> MAHHHHHHMTALLIRNVRTGADDALDILIEGDRIARTGPSLDAPPGCAIEEGAGAIALPGLVEGHTHLDKTHWGMPWYRNAVGPRLVDRIENERHYRATSGHDAGAASLALARAFLAAGTTRIRTHVDVDTDAGLRHLHRVL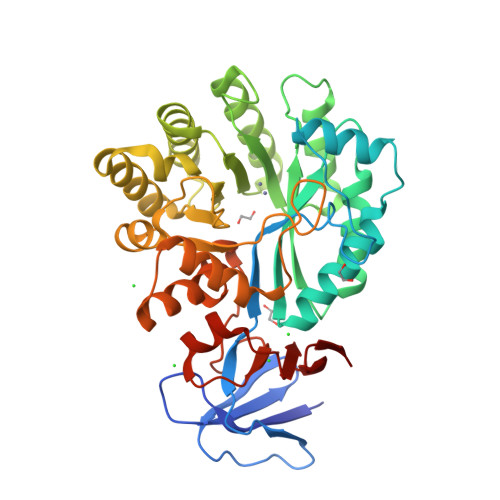DTRETLRGQVEIQIVAFPQSGVLKRPGTDALLADALAAGADLLGGLDPCAIEGDPVKAVDVLFGIAERYGRGLDLHLHERGSMGAYSLDLILQRTAALGMQHKVTISHAFCLGDLAERERDALLARMAELGVAVVTTAPAAVPVPSVLACRAAGVTVIGGNDGVRDTWTPYGSPDMLERAMLIAMRNDFRRDDALEVALECVTHGAARGCGFDAYGLQPGARADVVLVDAMTLAEAVVARPVRRLVVSSGKIVARNGALV>MMAFYDSIVENYHRDAVRGQAYSLVEKLAPLDQAGRQRQLEDWRPHYGLELSLTDARQAKLTQEEQAL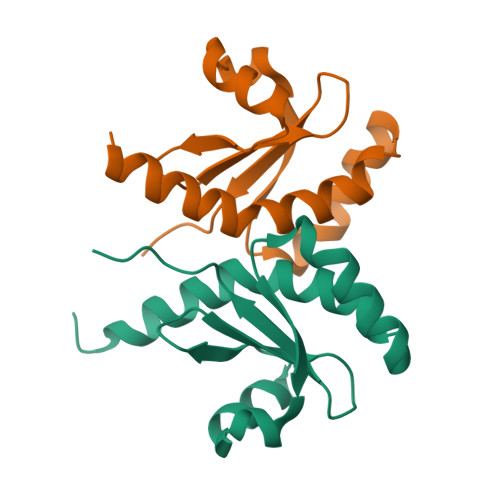LDKNLLVVREDFTEFISRIDAGPQLLDIKLPPEPSLT[2x]> MKIYRPLWEDGAFLMPQQFQQQAAWDVHLADSVARMGLAHPWGVVAAEFDDSLLPLSRLNATRLIVRFPDGTLIDTERADNLPPVCDLSTVSDRSLVDIVLALPLLNANGGNLDNGSESERPRRWKSERVNVQELAGHEQSEVAVLRHNLTLRMAHQENAAWLTCPVTRLVRDAQGQWC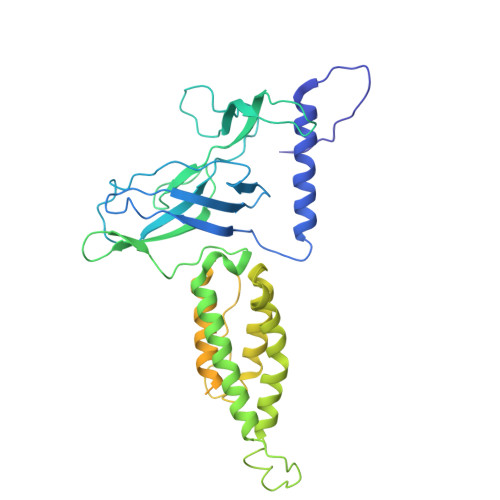RDPRFIPPLLTLSASPSLMTELLELLHHLQARRQRLMSMRRENNARLADFAVADVSLFWLLNALNSAEPVLKELLDMPYRHPELLYRELARLAGSLLTFSLEHNVDAVPAYHHETPENVFPPLLSLLNRLLEASLPSRVVFIELKQKGVMWEGALHDARLREGADFWLSVRSSMPGHELQTKFPQLCKAGSPDDVSEVVNVALSGVIIRPVTHVPAAIPLRLENQYFALDLSTDAARAMLDAGRCTFYTPASLGDVKLELFAVLRT pentalenolactone | C15 H16 O5 | 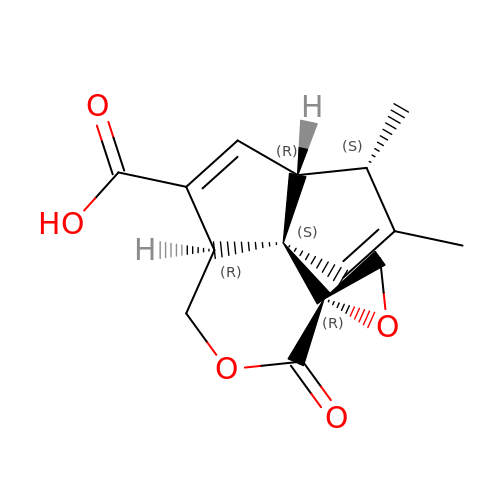NUPNVWUYFVEAIT-UJJBCWTCSA-N>[2x]MKKAVINGEQI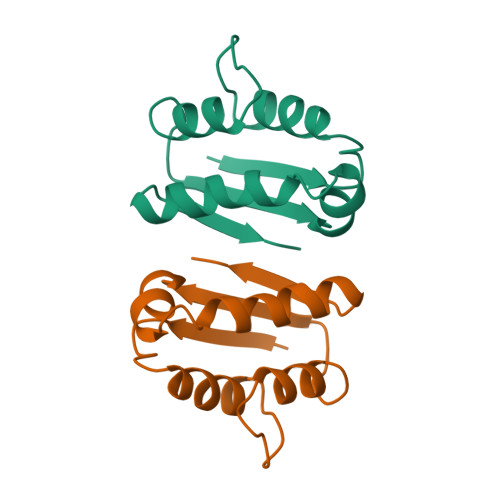RSISDLHQTLKKELALPEYYGENLDALWDCLTGWVEYPLVLEWRQFEQSKQLTENGAESVLQVFREAKAEGADITIILS>[6x]MKAFILA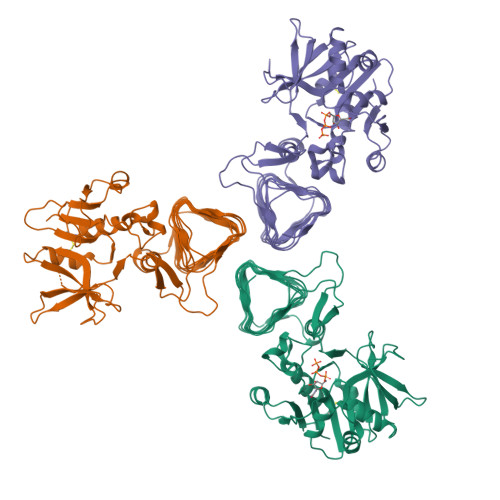AGSGERLEPITHTRPKAFVPILSKPLIEYQIEYLRKCGIRDITVIVSSKNKEYFEKKLKEISIVTQKDDIKGTGAAILSAKFNDEALIINGDLFFSNEKEICNIITLKENAIIGVKVSNPKDYGVLVLDNQNNLSKIIEKPEIPPSNLINAGIYKLNSDIFTYLDKISISERGELELTDAINLMAKDHRVKVIEYEGYWMDIGKPWNIIDVNKWALDNLVFSQNLGNVEDNVKIKGKVIIEEDAEIKSGTYIEGPVYIGKGSEIGPNSYLRPYTILVEKNKIGASVEVKESVIMEGSKIPHLSYVGDSVIAEDVNFGAGTLIANLRFDEKEVKVNVKGKRISSGRRKLGAFIGGHVRTGINVTILPGVKIGAYARIYPGAVVNRDVGYGEFFKVLEHHHHHH> MIMDKSIPKATAKRLSLYYRIFKRFNTDGIEKASSKQIADALGIDSATVRRDFSYFGELGRRGFGYDVKKLMNFFAEILNDHSTTNVMLVGCGNIGRALLHYRFHDRNKMQISMAFDLDSNDLVGKTTEDGIPVYGISTINDHLIDSDIETAILTVPSTEAQEVADILVKAGIKGILSFSPVHLTLPKDIIVQYVDLTSELQTLLYFM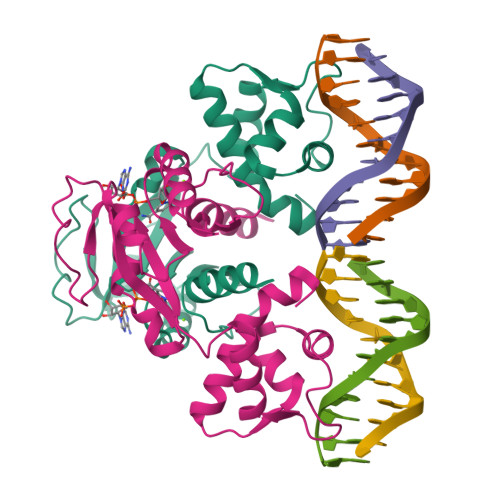NQQR> MPLYELLMLAKPSLPRAEMVALIKGLGDLVYRNGGFVTSLKSFGDQH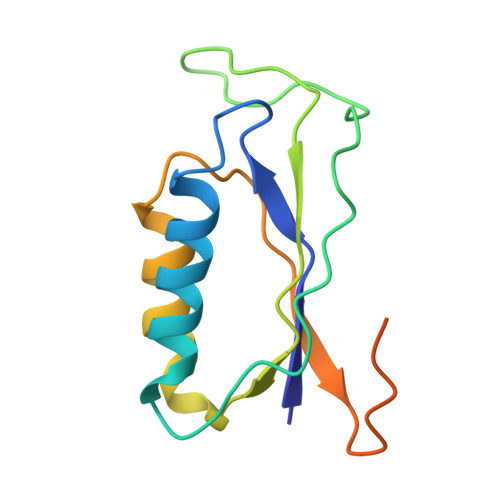LAYDLRRPFEKYDRAHIWQMDFVSSVDAIKPLDHGLHVNNTVLRWVLVKRPMSDKSAAAPAAATQAVEAIAQPQR Nucleoside diphosphate kinase A (NME1) is a multifunctional enzyme that was found to be pyrophosphorylated on Thr94 in human cells. A major role of NME1 is the synthesis of nucleoside triphosphates, other than ATP. NME1 catalyses this process by transferring the γ-phosphoryl group from ATP to a nucleoside diphosphate (NDP) via an active-site phosphohistidine intermediate. Oligophosphorylation was critically dependent on the catalytic histidine residue His118, and cryogenic electron microscopy analysis of the modified proteins suggests an intramolecular phosphoryl transfer mechanism.

For this, purified pS94-NME1 and ppS94-NME1 were vitrified, and cryo-EM datasets were recorded and refined to final resolutions of 2.8 Å for pS94-NME1 and 3.3 Å for ppS94-NME1. Notably, additional cryo-EM density at Ser94 was observed in both cases, which corresponds to the monophosphate or pyrophosphate group. The model for ppS94-NME1 indicates a more pronounced effect, and the distance between the β-phosphoryl group and the N1 of His118 amounts to only 4.5 Å. Further efforts to visualize the link between both side chains by comparing the maps at the same threshold showed that the densities for the His118 side chain and the pyrophosphate group are forming a bridge in the ppS94-NME1 map. The structural data suggest that the β-phosphoryl group of ppS94 is optimally placed (within 4.5 Å from His118) for a nucleophilic attack, and in closer proximity to the 1-pHis118 intermediate than the pS94 residue. This observation is corroborated by the biochemical data, which showed that ppS94-NME1 was much more competent to undergo oligophosphorylation, compared with pS94-NME1. The assay for ppS94-NME1 revealed that the pyrophosphoprotein exhibited almost no NDP kinase activity, even at a protein concentration of 1 µM. Interestingly, when ppS94-NME1 was incubated with ATP, an addition of four or five phosphoryl groups (+360 and +400 Da) became apparent. This ‘hyperphosphorylation’ was dependent on the catalytic His118 residue because the kinase-inactive mutant ppS94-NME1(H118F) did not undergo this modification.

>MHHHHHHMANCERTFIAIKPDGVQRGLVGEIIKRFEQKGFRLVGLKFMQASEDLLKEHYVDLKDRPFFAGLVKYMHSGPVVAMVWEGLNVVKTGRVMLGESNPADSKPGTIRGDFCIQVGRNIIHGSDSVESAEKEIGLWFHPEELVDYTSCAQNWIYE[6x]>MAASTPVVVDIHTHMYPPSYIAMLEKRQTIPLVRTFPQADEPRLILLSSELAALDAALADPAAKLPGRPLSTHFASLAQKMHFMDTNGIRVSVISLANPWFDFLAPDEAPGIADAVNAEFSDMCAQHVGRLFFFAALPLSAPVDAVKASIERVKNLKYCRGIILGTSGLGKGLDDPHLLPVFEAVADAKLLVFLHPHYGLPNEVYGPRSEEYGHV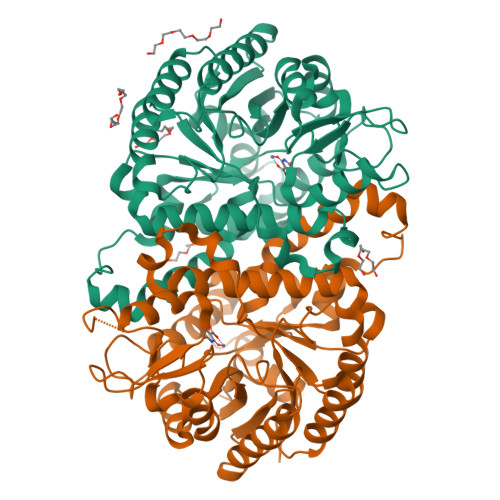LPLALGFPMETTIAVARMYMAGVFDHVRNLQMLLAHSGGTLPFLAGRIESCIVHDGHLVKTGKVPKDRRTIWTVLKEQIYLDAVIYSEVGLQAAIASSGADRLMFGTAHPFFPPIEEDVQGPWDSSRLNAQAVIKAVGEGSSDAAAVMGLNAVRVLSLKAE[4x]> SSLDDKPQFPGASAEFIDKLEFIQPNVISGIPIYRVMDRQGQIINPS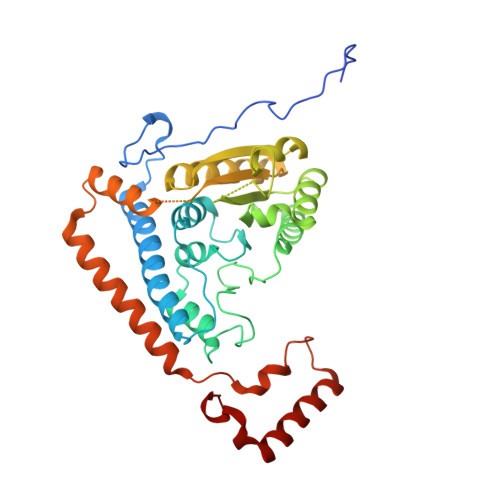EDPHLPKEKVLKLYKSMTLLNTMDRILYESQRQGRISFYMTNYGEEGTHVGSAAALDNTDLVFGQYREAGVLMYRDYPLELFMAQCYGNISDLGKGRQMPVHYGCKERHFVTISSPLATQIPQAVGAAYAAKRANANRVVICYFGEGAASEGDAHAGFNFAATLECPIIFFCRNNGYAISTPTSEQYRGDGIAARGPGYGIMSIRVDGNDVFAVYNATKEARRRAVAENQPFLIEAMTYRIGHASTSDDSSAYRSVDEVNYWDKQDHPISRLRHYLLSQGWWDEEQEKAWRKQSRRKVMEAFEQAERKPKPNPNLLFSDVYQEMPAQLRKQQESLARHLQTYGEHYPLDHFDK>RKLPVFKSLRHMRQVLGAPSFRMLAWHVLMGNQVIWKSRDVDLVQSAFEVLRTMLPVGCVRIIPYSSQYEEAYRCNFLGLSPHVQIPPHVLSSEFAVIVEVHAAARSTLHPVGAEDDQSLSKYEFVVTSGSPVAADRVGPTILNKIEAALTNQNLSVDVVDQALVALKEEWMNK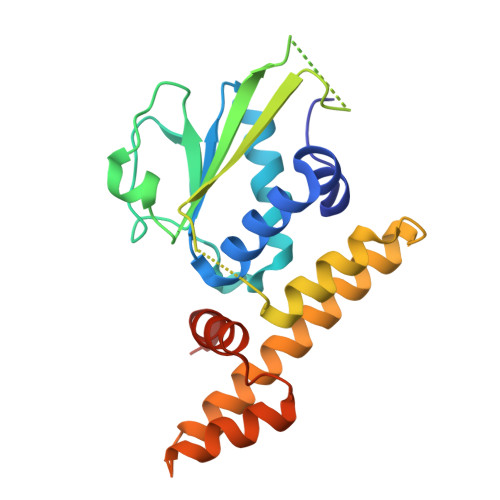VKVLFKFTKVDSRPKEDTQKLLSILGASEEDNVKLLKFWMTGLSKTYKSHLM[2x]> MSEKPTLF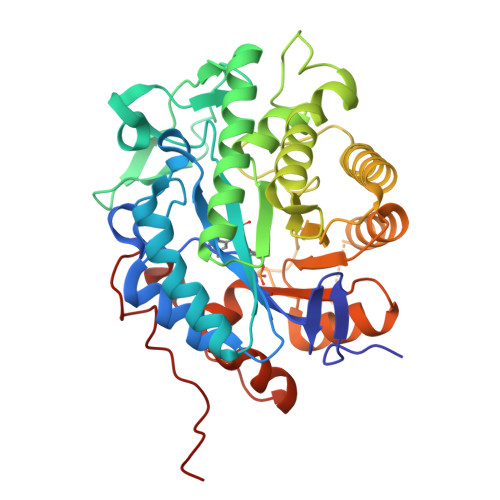SAYKMGKFNLSHRVVLAPMTRCRAINAIPNEALVEYYRQRSTAGGFLITEGTMISPSSAGFPHVPGIFTKEQVEGWKKVVDAAHKEGAVIFCQLWHVGRASHQVYQPGGAAPISSTSKPISKKWEILLPDATYGTYPEPRPLAANEILEVVEDYRVAAINAIEAGFDGIEIHGAHGYLLDQFMKDGINDRTDEYGGSLENRCKFILQVVQAVSAAIGTDRVGIRISPAIDHTDAMDSDPRSLGLAVIERLNKLQFKLGSRLAYLHVTQPRYTADGHGQTEAGANGSEEEVAQLMKTWRGAYVGTFICCGGYTRELGLQAVAQGDADLVAFGRYFVSNPDLVLRLKLNAPLNRYDRATFYTHDPVVGYTDYPSLDKGSLL> MTRETERFPAREFQRD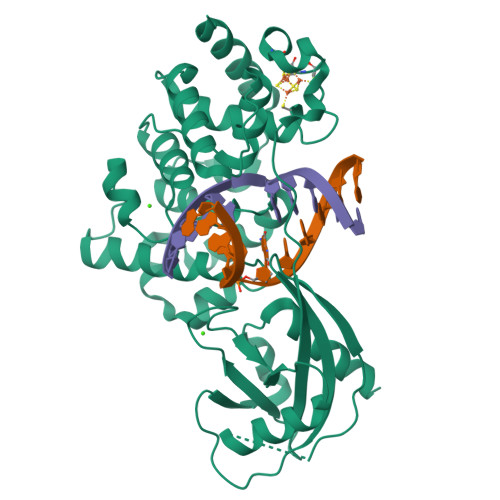LLDWFARERRDLPWRKDRDPYKVWVSEVMLQQTRVETVIPYFEQFIDRFPTLEALADADEDEVLKAWEGLGYYSRVRNLHAAVKEVKTRYGGKVPDDPDEFSRLKGVGPYTVGAVLSLAYGVPEPAVDGNVMRVLSRLFLVTDDIAKPSTRKRFEQIVREIMAYENPGAFNEALIELGALVCTPRRPSCLLCPVQAYCQAFAEGVAEELPVKMKKTAVKQVPLAVAVLADDEGRVLIRKRDSTGLLANLWEFPSCETDGADGKEKLEQMVGEQYGLQVELTEPIVSFEHAFSHLVWQLTVFPGRLVHGGPVEEPYRLAPEDELKAYAFPVSHQRVWREYKEWASGVRPPP>[4x]GSHMQVTPRRNVLQKRPVIVKVLSTTKPFEYETPEMEKKIMFHATVATQTQFFHVKVLNTSLKEKFNGKKIIIISDYLEYDSLLEVNEESTVSEAGPNQTFEVPNKIINRAKET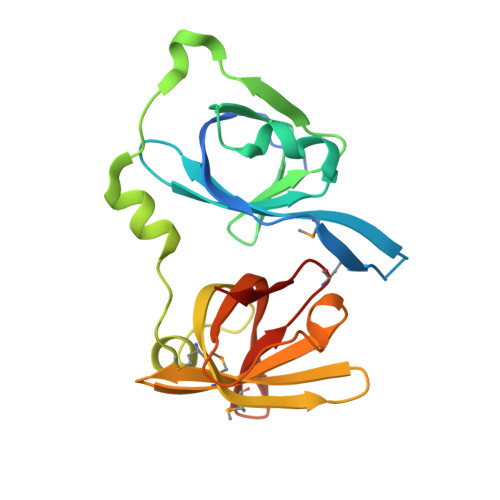LKIDILHKQASGNIVYGVFMLHKKTVNQKTTIYEIQDDRGKMDVVGTGQCHNIPCEEGDKLQLFCFRLRKKNQMSKLISEMHSFIQIKKKTN>CGCGCG[3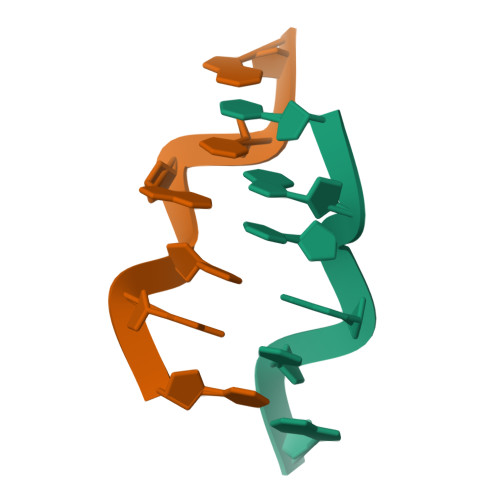x]> GKRPINPTDQSSYIVDSVTVKNGSIHLYFDKAGQKTYERHSLSHFVNLDNLRANNTKGSLPINVIVFDGKSKCEESSAKSASVYYSQLMCQPILLLDQALVSDVGDSAEVAVKMFDAYVNTFSSTFNVPMEKLKTLVATAEAELAKNVSLDNVLSTFISAARQGFVDSDVETKDVVECLKLSHQSDIEVTGDSCNNYMLTYNKVENMTPRDLGACIDCSARHINAQVAKSHNIALIWNVKDFMSLSEQLRKQI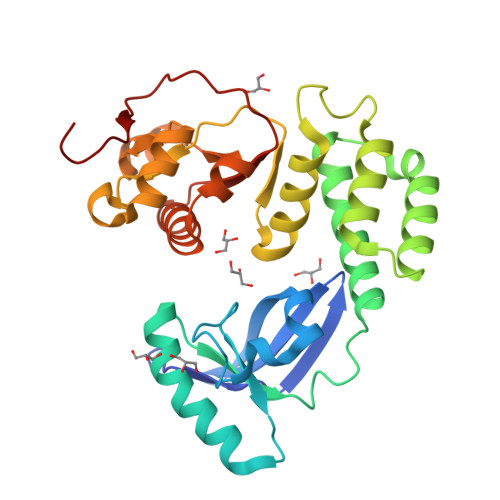RSAAKKNNLPFKLTCATTRQVVNVVTTKIALKGG> SERLLDELTLEGVARYMQSERCRRVICLVGAGISTSAGIPDFRSPSTGLYDNLEKYHLPYPEAIFEISYFKKHPEPFFALAKELYPGQFKPTICHYFMRLLKDKGLLLRCYTQNIDTLERIAGLEQEDLVEAHGTFYTSHCVSASCRHEYPLSWMKEKIFSEVTPKCEDCQSLVKPDIVFFGESLPARFFSCMQSDFLKVDLLLVMGTSLQVQPFASLISKAPLSTPRLLINKEKAGQSDPFLGMIMGLGGGMDFDSKKAYRDVAWLGECDQGCLALAELLGWKKELEDLVRREHASIDAQS

Human sirtuin 2 (SIRT2) is an NAD+ dependant enzyme that has been linked to the pathogenesis of various diseases, making it a promising target for pharmaceutical intervention. Sirtuins, belonging to class III histone deacetylases, constitute a family of highly conservative NAD+-dependant proteins that are involved in the regulation of various biological processes such as metabolism, aging, inflammation and oxidative stress. Although sirtuins were initially recognised solely for their deacetylation activity, recent studies unveiled a broader catalytic scope that includes desuccinylation, demalonylation, demyristoylation4 and ADP-ribosylation. To this end, we expressed human SIRT2 56-356 as a N-terminal His6-SUMO fusion in Escherichia coli and purified the protein via affinity and size exclusion chromatography with tag removal in between.

The most potent and subtype selective SIRT2 inhibitor 29 (RW-78) exhibits an IC50 of 26 nM, which outperforms its lead structure 24a (IC50 = 79 nM) by a factor of 3. Additionally, the chlorine or iodine atom engages in halogen–π-interactions with F235. The spacing between the chlorine atom of 29 and the centroid of the π-system of F235 (3.6 Å) matches the average distance of C–Cl⋯π-bonds (3.854 Å),50 explaining the high potency of 29. Contrary to our design, 29 and 31 do not engage in interactions with the SIRT2 co-factor NAD+ but stabilize the enzyme in an inactive state. In addition, by interacting with the inhibitor, F96 and R97 move into the NAD+-binding pocket, displacing the co-factor and prohibiting NAD+-binding. Therefore, the determined structures do not show electron densities for the co-factor, although 5 mM NAD+ was included in the crystallization screens. Notably, the NAD+ displacement is supported by thermal shift assays, which revealed that 29 increases the melting temperature of SIRT2 independently of NAD+. Compound 29 showed high target engagement with an EC50 value of 15 nM, validating our data obtained from in vitro inhibition studies.> IPSRILTRSQLRDVVASSHLLQSEFMEIPMNFVDPKEIDIPRHGTKNRYKTILPNPLSRVCLRPKNVTDSLSTYINANYIRGYSGKEKAFIATQGPMINTVDDFWQMVWQEDSPVIVM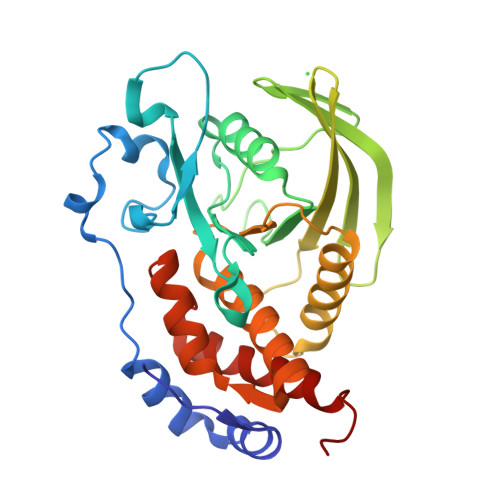ITKLKEKNEKCVLYWPEKRGIYGKVEVLVISVNECDNYTIRNLVLKQGSHTQHVKHYWYTSWPDHKTPDSAQPLLQLMLDVEEDRLASQGRGPVVVHCSAGIGRTGCFIATSIGCQQLKEEGVVDALSIVCQLRMDRGGMVQTSEQYEFVHHALCLYESRLSAET[(2~{R},3~{S},4~{R},5~{R})-5-(2-azanyl-6-oxidanylidene-1~{H}-purin-9-yl)-3,4-bis(oxidanyl)oxolan-2-yl]methoxy-(3-methyl-1~{H}-pyrazol-4-yl)phosphinic 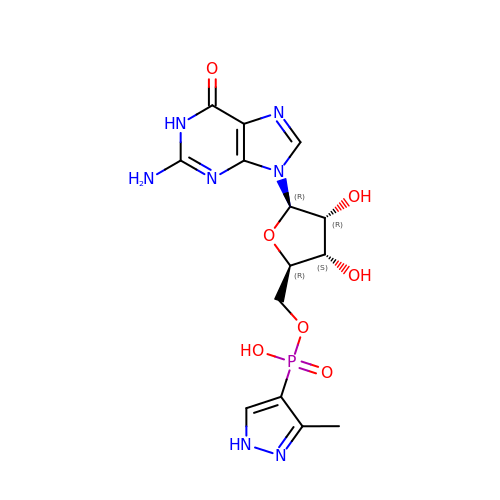acid | C14 H18 N7 O7 P | KSGRBDIXLOOOHG-ZRFIDHNTSA-N>GSHMDSEIQMENLVERKHHRLARSERSGISDRDAKPTASIRDQLHTIVYRYPPTYVLSSEEQDLVWKFRFYLSSHKKALTKFLKCINWKLEDEVTQALWMLANWAPMDVEDALELLSPTFTHPQVRKYAVSRLAQAPDEDLLLYLLQLVQALKYEDPRHIVHLHGCIFPERDVVRSILDDNGSLLDQSSLSDLSATSSGLHASVIPANQRAASVLAAIKSDKSVSPGSAGGSGSGGQGSVALPNPSAPATPGSSSLPCDSNSNALMLAEGISFGSVPANLCTFLIQRACTNATLANYFYWYLSIEVEEVESVRKQDERAHDMYAMVLKMFLKVLENGNFNLRGIFYNLRKQRRFIDELVKLVKLVAKEPGNRNKKTEKFQKLLAEQDMFKVNFTNFEPIPFPLDPEIYITKIVPMRTSLFKSALMPAKLTFVTSIAHHEYAAIFKHGDDLRQDQLILQMITLMDKLLRRENLDLKLTPYKVLATSSKHGFLQYVDSCTVAEVLAREGNIHNFFRKHHPCDNGPYGISAEVMDTYIKSCAGYCVITYLLGVGDRHLDNLLLTTNGKLFHIDFGYILGRDPKPMPPPMKLSKEMVEAMGGISSEHHHEFRKQCYTAYLHLRRHA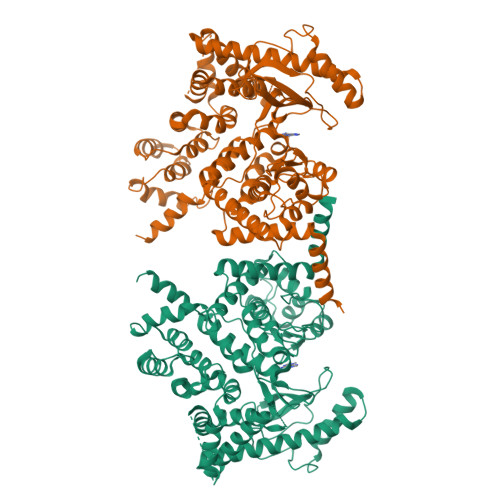NVMLNLFSLMVDATVPDIALEPDKAVKKVEENLQLGLTDEEAVQHLQSLLDVSITAVMPALVEQIHRFTQYWRK[2x]1-[4-chloranyl-3-(trifluoromethyl)phenyl]-3-[[(2R,3S)-5-[5-methyl-2,4-bis(oxidanylidene)pyrimidin-1-yl]-3-oxidanyl-oxolan-2-yl]methyl]thiourea 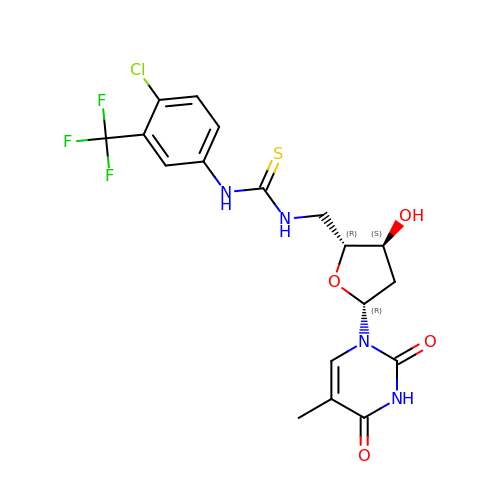| C18 H18 Cl F3 N4 O4 S | IJDGQXGQAWBJEG-BFHYXJOUSA-N>MKLSARNQLAGKVVSIKEGAVNGIVVLDIGGGNQISSTISMDSIRELGLQVGSDAYA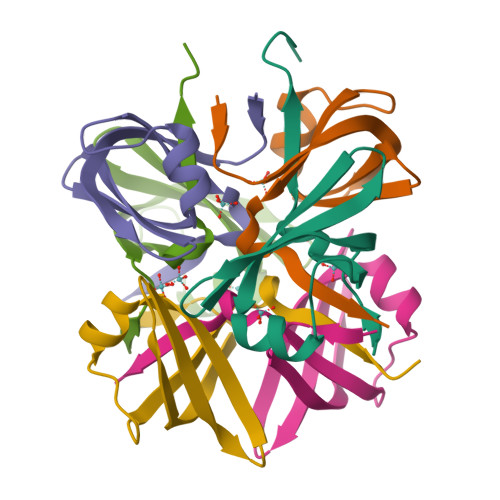VIKATSVMIGIDDWSHPQFEK[12x]> NLSLSQSNFSADTYKSFIKNLRKQLTIGASYGSAGIPILKHSVPICERFLLVDLTNGDNETITLAINVEDAGFAAYRAADRSYFFQNAPPIASYVIFTDTNQNIMNFNNTFESIEIVGGTTRSETPLGIMHFEASIFHLFVHDENYVPTSFLVLIQMVLEAAKFKFI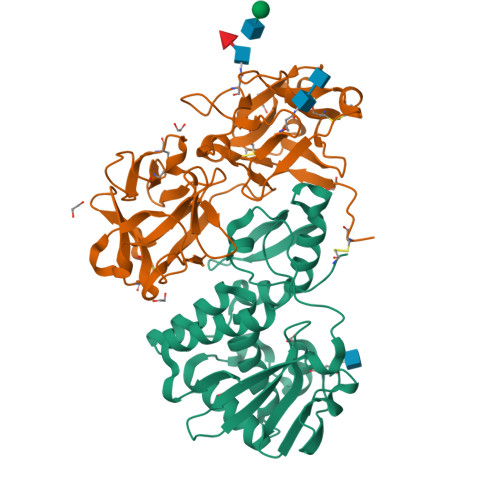EQKVIHSIMDMEDFTPGLAMLSLEENWTQLSLQLQASESLNGVFGDSVSLYNSMDEPIGVDSMYYPILTANMAFQLYQCP;> EQCSPQQRTTRISGRDGLCVDVYGALTADGSRVILYPCGQQQNQQWTFYPDNTIRSLGKCLATSALSSGSNVVITNCDYLRYDDGWMVSSSGTMMNKSSHLVLTANAATSRTNLTGENNVFAAKQAWRIGNYVEPIVTTIIGLRHMCLEATDNDTNVWLESCVKNKTKQYWALYSDDTIRVNNNRNLCVSSSTDSSSKLIVIRRCDGSINQRWVFTPQGTISNPGYEAVMDVAQNDVYLKKIVLSSATDKGNGQQWTVFY>[2x]MKQLSVSLAILCAVATSEAFAADELQQRAQGLFKPVPAKAPTLKGNPASPVKVELGKMLYFDPRLSASHLISCNTCHNVGLGGGDLQATSTGHGWQKGPRNAPTVLNSVFNTAQFWDGRAKDLAEQAKGPVQASVEMNNTP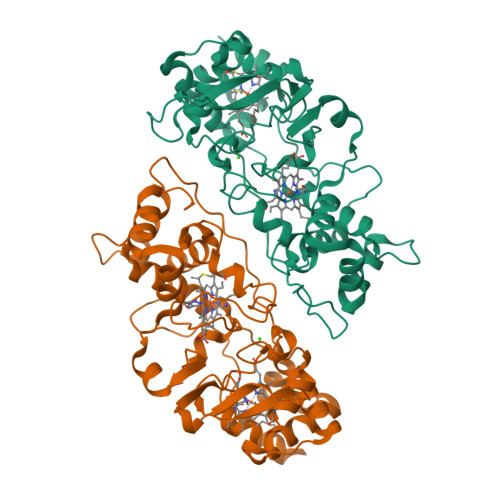DQVVKTLNSIPDYVALFKKAFPGEKDPVTFDNMAKAIEVFEATLITPDSPFDQYLKGKKKALDGKQTAGLKLFLDKGCVACHGGLNLGGTGYFPFGVVEKPAENILPLGDKGRFAVTNTAKDEYVFRAPSLRNVAITYPYFHSGVVWSLKEAVAVMGSAQFGIKLSDDESEAIAAFLGSLTGKQPKVVYPIMPASTDATPRPRL>[2x]MASMTG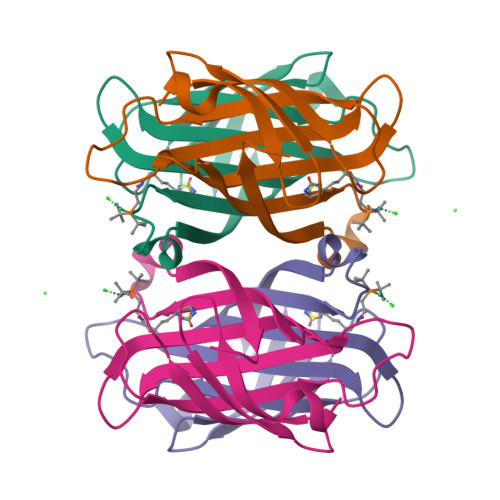GQQMGRDEAGITGTWYNQLGSTFIVTAGADGALTGTYESAVGNAESRYVLTGRYDSAPATDGSGTALGWTVAWKNNYRNAHSATTWSGQYVGGAEARINTQWLLTYGTTEANAWESTLVGHDTFTKVKPSAASIDAAKKAGVNNGNPLDAVQQ>AVGNATQPLLVVEDSDEDFSTFQRLLQREGVVNPIYRCITGDQALDFLYQTGSYCNPDIAPRPAVILLDLNLPGTDGREVLQEIKQDEVLKKIPVVIMTTSSNPKDIEICYSYSISSYIVKPLEIDRLTETVQTFIK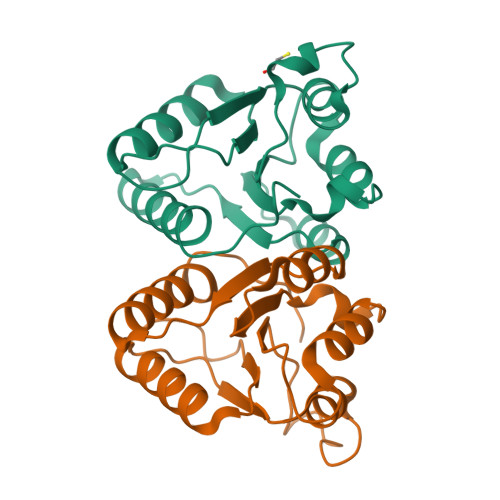YWLDIVVLPEMG[2x]(5R,7S)-8-benzyl-4-(cyclohexylamino)-1-(3-fluorophenyl)-7-methyl-1,3,8-triazaspiro[4.5]dec-3-en-2-one 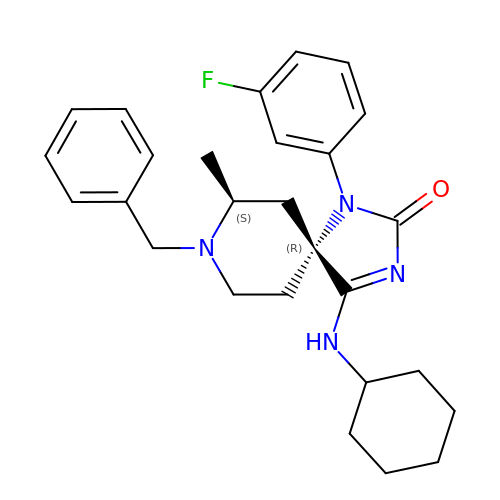| C27 H33 F N4 O | YNODVOARUZZRMG-CCLHPLFOSA-N> GSSGSSGMSNPNPFQTTLGTDAQWVVFAVMALAAIVFSIAVQFRPLPLRLTYYVNIAICTIAATAYYAMAVNGGDNKPTAGTGADE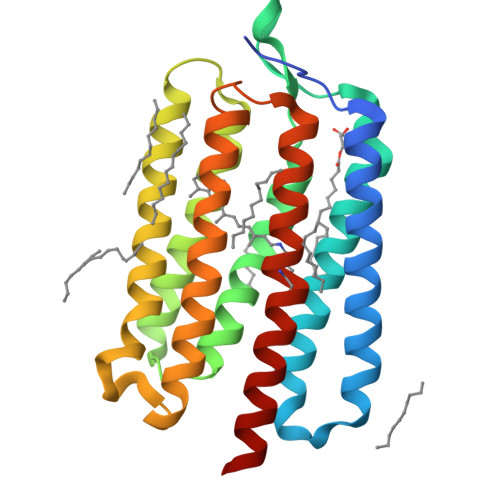RQVIYARYIDWVFTTPLLLLDLVLLTNMPATMIAWIMGADIAMIAFGIIGAFTVGSYKWFYFVVGCIMLAVLAWGMINPIFKEELQKHKEYTGAYTTLLIYLIVLWVIYPIVWGLGAGGHIIGVDVEIIAMGILDLLAKPLYAIGVLITVEVVYGKLG> GCUUCAACAACCCCGUAGGUGGGGACGAAAGUCAGCGCACCUACUGGAGCC

Riboswitches are gene regulatory elements that are frequently found in the 5′-untranslated regions of bacterial mRNAs (1–6). Only very recently, the nadA RNA motif has been assigned to function as a riboswitch which regulates the expression of genes involved in biosynthesis of the enzyme cofactor nicotinamide adenine dinucleotide (NAD+). Although the cofactor is ubiquitous, this riboswitch appears to be rather rare and has the special feature of a tandem aptamer architecture. Here, we report crystal structures of the first, as well as the second domain of the NAD+ riboswitch, both individually bound to NAD+.

The RNA adopts a pseudoknot scaffold in ‘Y-shape’, in which stems P1b, P1a and P1 form a co-axial long helix, with integrated base pairs from the internal bubble J2. The junctional loop J1 (residing between P1 and P1a) zippers up and forms a long-distance interaction with J2 (residing between stems P1a and P1b). NAD+ is bound at the intersection of stem P1 and the junction loop J1, employing a type-I A minor base triple. Importantly, C13 and C14 from J1 hydrogen bond with G38 and G36 from J2, respectively, forming two regular Watson–Crick base pairs. All these junction interactions including the long-distance pairing (G38-C13 and G36-C14) stabilize the overall fold, and simultaneously, position A8 of J1 as a key recognition element for NAD+ in the RNA binding pocket. The surface representation of the binding pocket shows that it is the ADP moiety of NAD+ that interacts intensively, with the nucleobase deeply buried into a cavity and the pyrophosphate nestling up the RNA surface, while the NMN moiety of NAD+ points outwards without any obvious RNA interactions. In more detail, the adenine base and the ribose of NAD+ form five hydrogen bonds with the minor groove edge of G47-C6 and hence generate a base triple, which is stacked between the base triple A8•A7-U46 and the non-canonical base pair of U5•G48. Three Mg2+ cations labeled M1, M2 and M3 were identified in the domain 1 binding pocket of the NAD+ riboswitch based on 2Fo-Fc and Fo-Fc maps guided by the coordination geometries, which were further validated by the observation of anomalous signals collected from Mn2+-soaked crystals. The three Mg2+ cations therefore determine the folding of J1, and hence, the NAD+ binding pocket, and one of them (M1) is key for mediating the interaction of the negatively charged pyrophosphate of ligand and selected phosphates of the aptamer, thereby creating a crucial recognition feature.>[4x]GAMSGEAPGIRKEMKDVTTKLGEAAQLSCQIVGRPLPDIKWYRFGKELIQSRKYKMSSDGRTHTLTVMTEEQEDEGVYTCIATNEVGEVETSSKLLLQATPQFHPGYPLKEKYYGAVGSTLR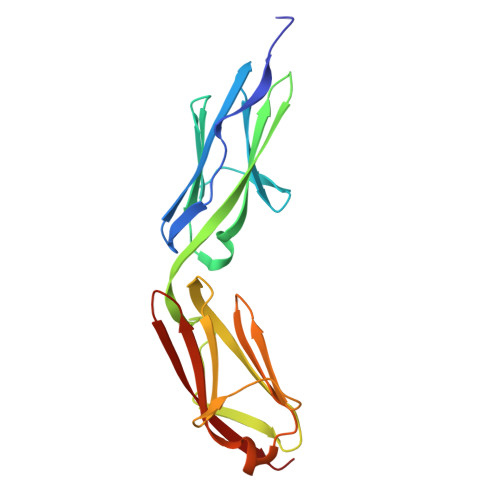LHVMYIGRPVPAMTWFHGQKLLQNSENITIENTEHYTHLVMKNVQRKTHAGKYKVQLSNVFGTVDAILDVEIQDK> MGPMANMEARNVMSGTWGELWLDGNKVAEVKKFQAKMEFTKEDIIIAGQMGTDTKYMGYKGKGSITLYHVSSRMHKLIGEKIKRGS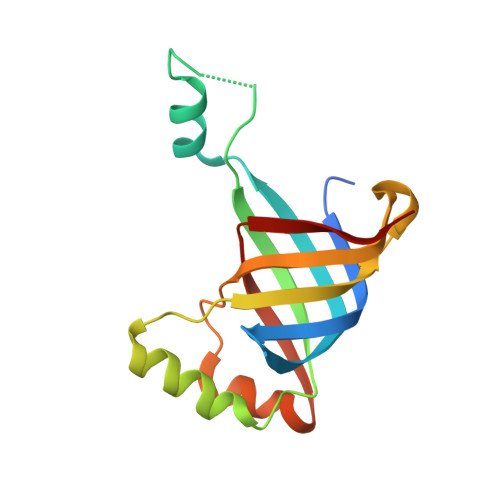EPRFVAISKLNDPDSYGAERIAVKNIAFDDLTLADWEVGVKGEIEAPFTFTEYDFLDII2-chloro-N-[1-(5-{[2-(4-fluorophenoxy)ethyl]sulfanyl}-4-methyl-4H-1,2,4-triazol-3-yl)ethyl]benzamide 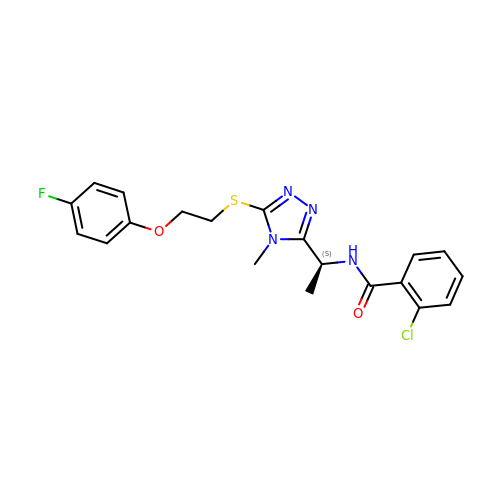| C20 H20 Cl F N4 O2 S | AJRDSERGUKXARL-ZDUSSCGKSA-N>SNAAMSQKHLQINQTFEELRLVTQDTENELKKLQQTQEYFIIQYQESLRIQAQFAQLAQLSPQERLSRETALQQKQVSLEAWLQREAQTLQQYRVELAEKHQKTLQLLRKQQTIILDDELIQWKRRQQLAGNGGPPEGSLDVLQSWCEKLAEIIWQNRQ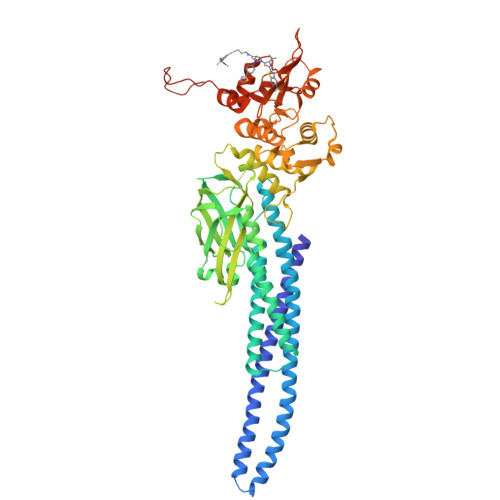QIRRAEHLCQQLPIPGPVEEMLAEVNATITDIISALVTSTFIIEKQPPQVLKTQTKFAATVRLLVGGKLNVHMNPPQVKATIISEQQAKSLLKNENTRNECSGEILNNCCVMEYHQATGTLSAHFRNMSLKRIKRADRRGAESVTEEKFTVLFESQFSVGSNELVFQVKTLSLPVVVIVHGSQDHNATATVLWDNAFAEPGRVPFAVPDKVLWPQLCEALNMKFKAEVQSNRGLTKENLVFLAQKLFNNSSSHLEDYSGLSVSWSQFNRENLPGWNYTFWQWFDGVMEVLKKHHKPHWNDGAILGFVNKQQAHDLLINKPDGTFLLRFSDSEIGGITIAWKFDSPERNLWNLKPFTTRDFSIRSLADRLGDLSYLIYVFPDRPKDEVFSKYYTPVLAKAVDGYVKPQIKQVVPE[2x]> MTATVLLEVPFSARGDRIPDAVAELRTREPIRKVRTITGAEAWLVSSYALCTQVLEDRRFSMKETAAAGAPRLNALTVPPEVVNNMGNIADAGLRKAVMKAITPKAPGLEQFLRDTANSLLDNLITEGAPADLRNDFADPLATALHCKVLGIPQEDGPKLFRSLSIAFMSSADPIPAAKINWDRDIEYMAGILENPNITTGLMGELSRLRKDPAYSHVSDELFATIGVTFFGAGVISTGSFLTTALISLIQRPQLRNLLHEKPELIPAGVEELLRINLSFADGLPRLATADIQVGDVLVRKG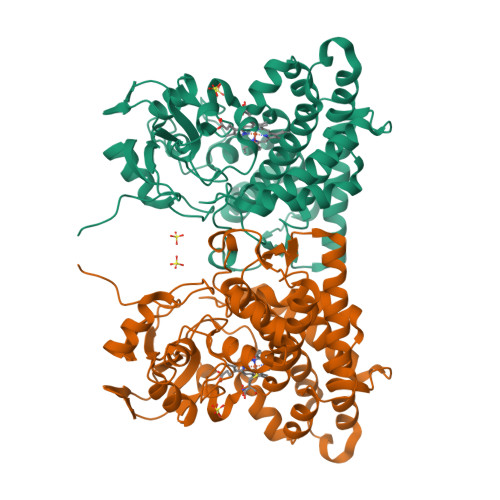ELVLVLLEGANFDPEHFPNPGSIELDRPNPTSHLAFGRGQHFCPGSALGRRHAQIGIEALLKKMPGVDLAVPIDQLVWRTRFQLRIPERLPVLW> MGQEGKGTCILVGGHEITSGLEVISSLRAIHGLQVEVCPLNGCDYIVSNRMVVERRSQSEMLNSVNKNKFIEQIQHLQSMFERICVIVEKDREKTGDTSRMFRRTKSYDSLLTTLIGAGIRILFSSCQEETADLLKELSLVEQRKNVGIHVPTVVNSNKSEALQFYLSIPNISYITALNMCHQFSSVKRMANSSLQEISMYAQVTHQKAEEIYRYIHYVFD;> MGHIVANEKWRGSQLAQEMQGKIKLIFEDGLTPDFYLSNRCCILYVTEADLVAGNGYRKRLVRVRNSNNLKGIVVVEKT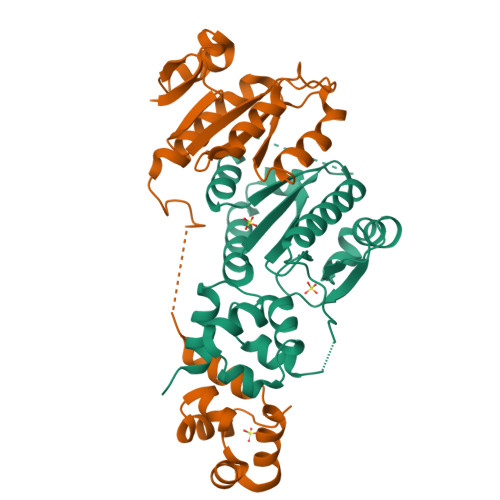RMSEQYFPALQKFTVLDLGMVLLPVASQMEASCLVIQLVQEQTKEPSKNPLLGKKRALLLSEPSLLRTVQQIPGVGKVKAPLLLQKFPSIQQLSNASIGELEQVVGQAVAQQIHAFFTQPRLEHHHHHH> MAWPKVQPEVNIGVVG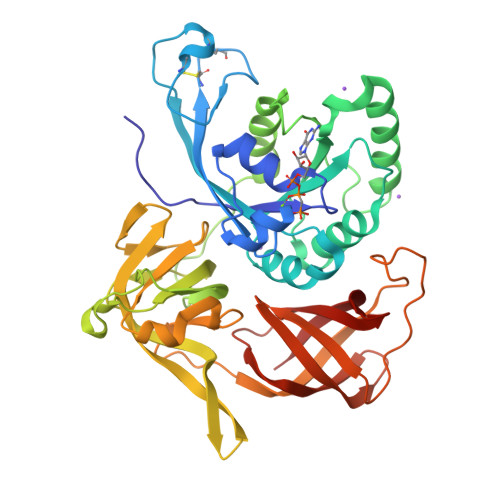HVDHGKTTLVQAITGIWTSKHSEELKRGMTIKLGYAETNIGVCESCKKPEAYVTEPSCKSCGSDDEPKFLRRISFIDAPGHEVLMATMLSGAALMDGAILVVAANEPFPQPQTREHFVALGIIGVKNLIIVQNKVDVVSKEEALSQYRQIKQFTKGTWAENVPITPVSALHKINIDSLIEGIEEYIKTPYRDLSQKPVMLVIRSFDVNKPGTQFNELKGGVIGGSIIQGLFKVDQEIKVLPGLRVEKQGKVSYEPIFTKISSIRFGDEEFKEAKPGGLVAIGTYLDPSLTKADNLLGSIITLADAEVPVLWNIRIKYNLLERVVGAKEMLKVDPIRAKETLMLSVGSSTTLGIVTSVKKDEIEVELRRPVAVWSNNIRTVISRQIAGRWRMIGWGLVEI>[2x]MGYLHRVVEGLKANAGGEALVSADRRLTGAETLEEIHRTARALAAQGLRPGDGVVTLHGNGVEAVVLRIAVQLLGCRYAGLRPVFATREKANFLAEAEAAAFVYQPDMADEAAELLREVPTPRVLSLGPAPLGEDLVALAGAQSAEPVEFTADERAATAVGFTGGTTGRAKGVCRAPFDLEACLDASLTIFGEGPWRFLVCI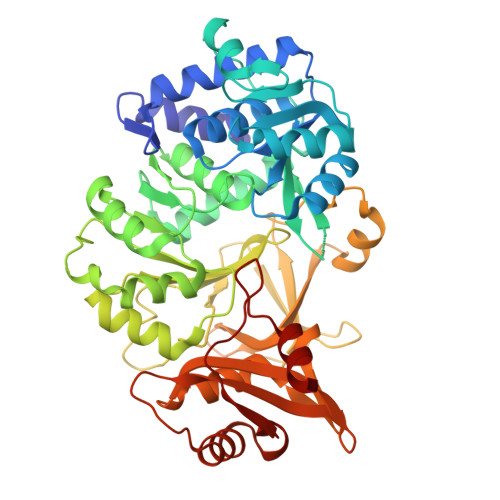PIADLGGEMAEWTLAAGGTVVLREDFEPADILATIGAERTTHVFCAPGWVYQLAEHPALADADLSSLTQIPYGGAPSTPARIADALEKLGRPLLVHCYGSQEGGWMTWLSAEDHVRADRYLLNSVGKALPGTEIAIRDQDGADLPVGTVGEVCVRSTMLMRGYWRLPELTAKTVRDGWLHTGDLGRLDTEGYLYLVDRAKDVIIVEAYNVYSQEVEHVLTGHPDVRYAAVVGVPDHDTTEAVYAAVVPAEGVGEIDVDELRALVRTTLGPVHEPKHLDVVDTIPTTPRGHPDKSALRTRWRA> GPPTERHFYHVLVKHKDVRRPSSLAPRNKGEKITRSRADAINLAQAILAQHKERKTWSLDEFVQVVRDFSECGSAK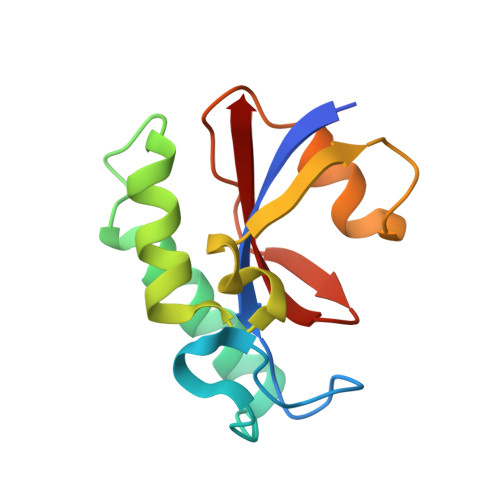RDGDLGMVESGTYTEGFDTVAFSLKSGEVSAPVETELGVHLIYRVE>[2x]MHHHHHHQIGWRREGIKYRRNELFLDVLESVNLLMSPQGQVLSAHVSGRVVMKSYLSGMPECKFGMNDKIVIEKQGKGTADETSKSGKQSIAIDDCT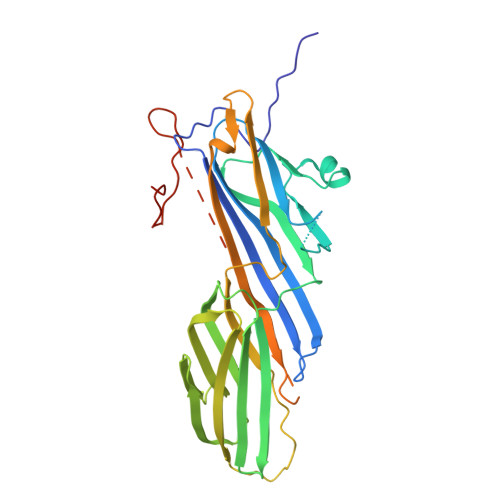FHQCVRLSKFDSERSISFIPPDGEFELMRYRTTKDIILPFRVIPLVREVGRTKLEVKVVIKSNFKPSLLAQKIEVRIPTPLNTSGVQVICMKGKAKYKASENAIVWKIKRMAGMKESQISAEIELLPTNDKKKWARPPISMNFEVPFAPSGLKVRYLKVFEPKLNYSDHDVIKWVRYIGRSGIYETRCGASGSAGSAGPSGAGSAGSAGPSAGSAGSAGSGSAGSAPGPDVDEEGYSIKPETNQNDTKENHFYSSSDSDSEDEE The periplasmic binding proteins (PBP) are a protein superfamily that serve as primary receptors for a diverse group of metabolic solutes in signaling, chemotaxis and metabolite transport systems in bacteria, eukaryotes and archaea. PBPs are comprised of two α/β domains connected by a flexible linker region that serves as a pivot point for the ligand induced hinge-bending motion that this protein superfamily is known for. Unlike other PBPs, the tmCBP binding site is bipartite, being composed of a typical PBP solvent excluded disaccharide binding site (subsite one) that is adjacent to an atypical large solvent filled cavity (subsite two) where three additional saccharide rings could be placed. The structure of tmCBP was solved in the presence of β(1,4) linked sugars, however the size of the tmCBP binding cavity and molecular modeling suggested additional glucan sugar linkages could be accommodated in both the disaccharide binding site and the solvent filled cavity. tmCBP is found in an operon that consists of an ABC transport system and an endoglucanase, the natural substrate of which has been predicted to be the algae-based storage polysaccharide laminarin.

The crystal structure of tmCBP complexed with LR2 was solved to a resolution of 2.05 Å by molecular replacement using the previously determined tmCBP structure. The final model consists of 582 amino acids, a larminaribiose molecule and 293 water molecules. The overall fold and conformation of the protein is similar to the structure of the cellobiose complexed protein (all atom RMSD= 0.4 Å). An extensive network of polar and non-polar amino acids and water molecules bind the LR2 ligand. A total of six tryptophan residues (Trp15, Trp380, Trp383, Trp426, Trp510 and Trp535) form van der Waals interactions with the two sugar rings. In total, ten hydrogen bonds can be formed with the first sugar ring. All but one hydrogen bond are directly formed with the protein, with the C6 hydroxyl being ligated by a single specifically bound water molecule, W20. For second sugar ring of the laminaribiose, only the C2 hydroxyl forms a direct hydrogen bond with the main chain carbonyl of Gly12, which also forms a hydrogen bond with the C2 hydroxyl of the first ring. The other six hydrogen bonds with the second ring are with water molecules. Unlike the other tmCBP structures that have been solved thus far, both the LR2 complex and the LR5 complex contain a pentagonal bipyrimidally-bound calcium ion.

> SLPREDTVYIGGALWGPATTWNLYAPQSTWGTDQFMYLPAFQYDLGRDAWIPVIAERYEFVDDKTLRIYIRPEARWSDGVPITADDFVYALELTKELGIGPGGGWDTYIEYVKAVDTKVVEFKAKEENLNYFQFLSYSLGAQPMPKHVYERIRAQMNIKDWINDKPEEQVVSGPYKLYYYDPNIVVYQRVDDWWGKDIFGLPRPKYLAHVIYKDNPSASLAFERGDIDWNGLFIPSVWELWEKKGLPVGTWYKKEPYFIPDGVGFVYVNNTKPGLSDPAVRKAIAYAIPYNEMLKKAYFGYGSQAHPSMVIDLFEPYKQYIDYELAKKTFGTEDGRIPFDLDMANKILDEAGYKKGPDGVRVGPDGTKLGPYTISVPYGWTDWMMMCEMIAKNLRSIGIDVKTEFPDFSVWADRMTKGTFDLIISWSVGPSFDHPFNIYRFVLDKRLSKPVGEVTWAGDWERYDNDEVVELLDKAVSTLDPEVRKQAYFRIQQIIYRDMPSIPAFYTAHWYEYSTKYWINWPSEDNPAWFRPSPWHADAWPTLFIISKKSDPQPVPSWLGTVDEGGIEIPTAKIFEDLQKAT>[2x]MLSG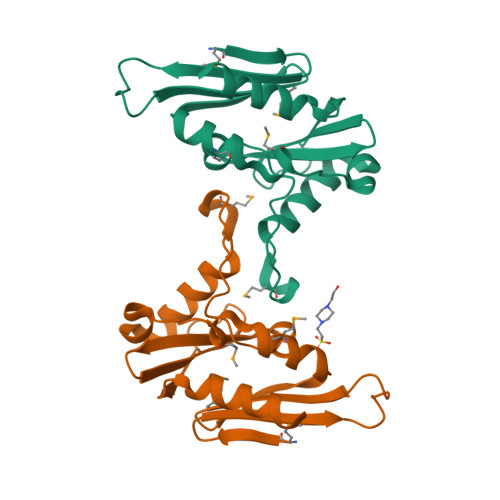NPHTFAIWCDAVESWSTPAFANGCLGYFMGGKLVWSSNSTLGVDLSMLSRLHCMRNTVEDAELFHISPEDAYRELCNRAFPSMDSGAESNDFTHLVSAESLSDEGYYIFLVEYDESAKLIYGFKENSREAGEVVLVRGEFQSVVRDVLAKSPKDFNAGSLAGHHHHHH>[2x]TQNNESAEADMQQQQSKEMSQEMETLMESIKKALEREIEQGAIEVENLGQQIVIRMREKGAFPEGSAFLQPKFRPLVRQIAELV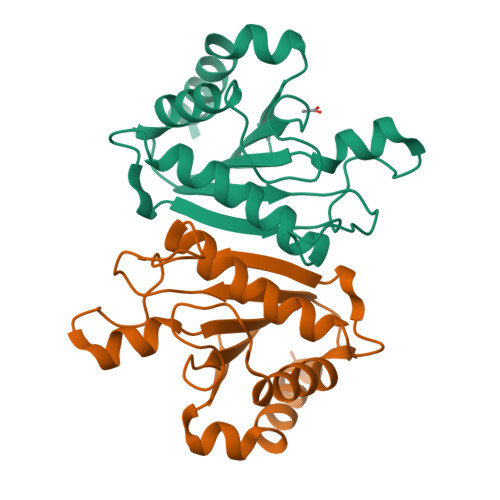KDVPGIVRVSGHTDNRPLDSELYRSNWDLSSQRAVSVAQEMEKVRGFSHQRLRVRGMADTEPLLPNDSDDNRALNRRVEISIMQGEPLYSEEVPVIQHHHHHH> QRCGSQGGGATCPGLRCCSIWGWCGDSEPYCGRTCENKCWSGERSDHRCGAAVGNPPCGQDRCCSVHGWCGGGNDYCSGGKCQYRCSS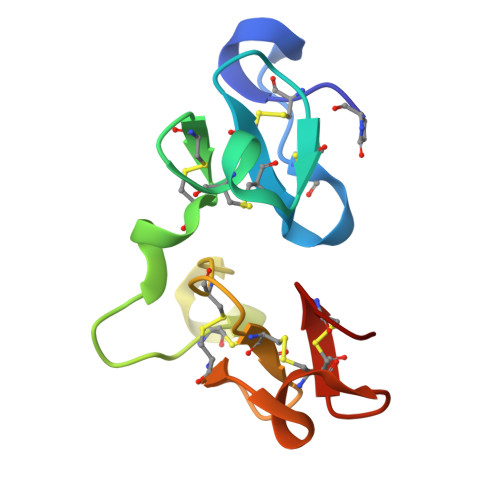S Taurodeoxycholate | C26 H45 N O6 S | 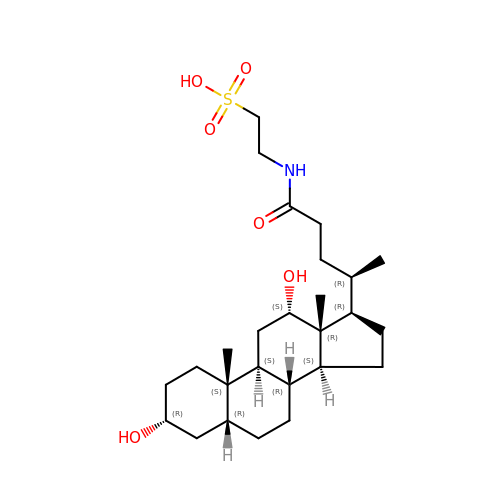AWDRATDZQPNJFN-VAYUFCLWSA-N> MDIAVQLVDSGGGTLQAGKSLRLSCAISGLAFDGGAMGSEHRLTAGAMGWFRQAPGKDREFVAAISPRTDETYYAESLEGRFSVSRDAAATMVFLQADNVRLDDTASYYCAADEDVTPRVMGVIPHADHWGQGTLVTVSSAAALEHHHHHH;> MAVQFVNKQFNYKDPVNGVDIAYIKIPNVGQMQPVKAFKIHNKIWVIPERDTFTNPEEGDLNPPPEAKQVPVSYYDSTYLSTDNEKDNYLKGVTKLFERIYSTDLGRMLLTSIVRGIPFWGGSTIDTELKVIDTNCINVIQPDGSYRSEELNLVIIGPSADIIQFECKSFGHEVLNLTRNGYGSTQYIRFSPDFTFGFEESLEVDTNPLLGAGKFATDPAVTLAHELIHAGHRLYGIAINPNRVFKVNTNAY;> YEMSGLEVSFEELRTFGGHDAKFIDSLQENEFRLYYYNKFKDIASTLNKAKSIVGTTASLQYMKNVFKEKYL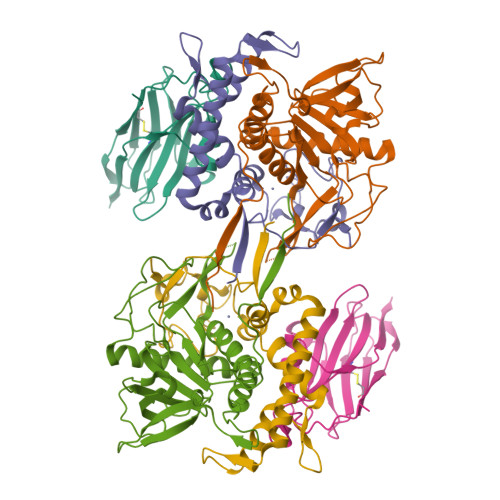LSEDTSGKFSVDKLKFDKLYKMLTEIYTEDNFVKFFKVLNRKTYLNFDKAVFKINIVPKVNYTIYDGFNLRNTNLAANFNGQNTEINNMNFTKLKNFTGLFEF>GSHMESFLLSKVSFVIKKIRLEKGMTQEDLAYKSNLDRTYISGIERNSA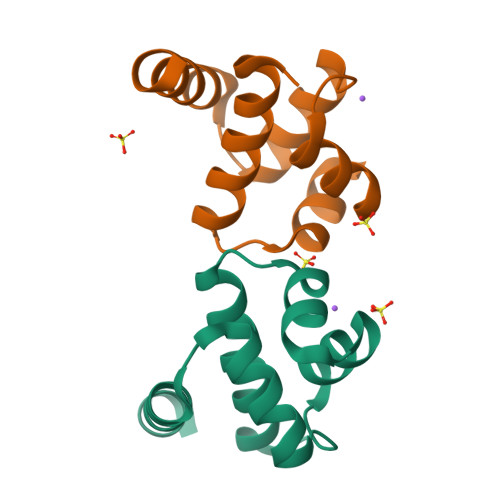NLTIKSLELIMKGLEVSDVVFFEMLIKEILKHD[2x]> GSPEFMGEQPIFSTRAHVFQIDPNTKKNWVPTSKHAVTVSYFYDSTRNVYRIISLDGSKAIINSTITPNMTFTKT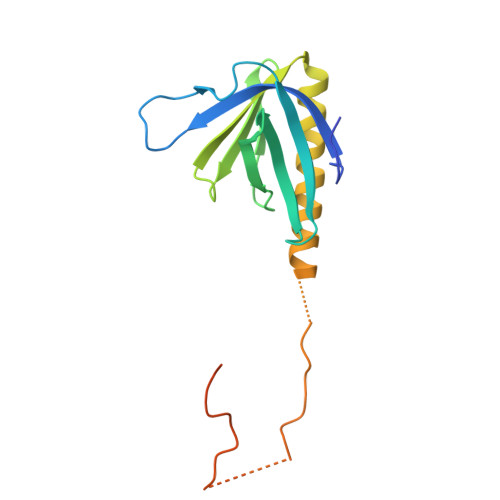SQKFGQWADSRANTVYGLGFSSEHHLSKFAEKFQEFKEAARLAKEKSQEKMELTSTPSQESAGGDLQSPLTPESINGTDDERTPDVTQNSEPR> RGKGG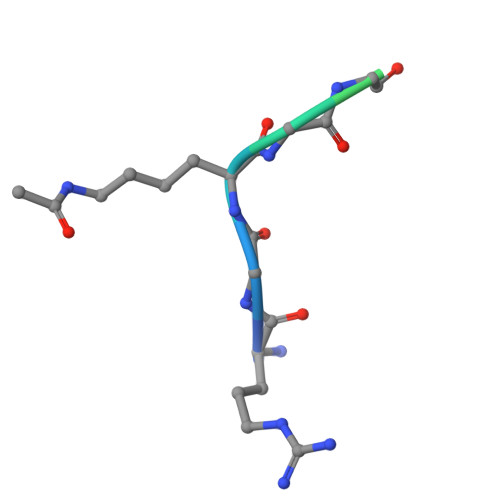KGLGKGGAY>GAMETITVPTPIKQIFSDDAFAETIKDNLKKKSVTDAVTQNELNSIDQIIANNSDIKSVQGIQYLPNVTKLFLNGNKLTDIKPLANLKNLGWLFLDENKVKDLSSLKDLKKLKSLSLEHNGISDINGLVHLPQLESLYLGNNKITDITVLSRLTKLDTLSLEDNQISDIVPLAGLTKLQNLYLSKNHISDLRALAGLKNLDVLELFSQECLNKPINHQSNLVVPNTVKNTDGSLVTPEIISDDGDYEKPNVKWHLPEFTNEVSFIFYQPVTIGKAK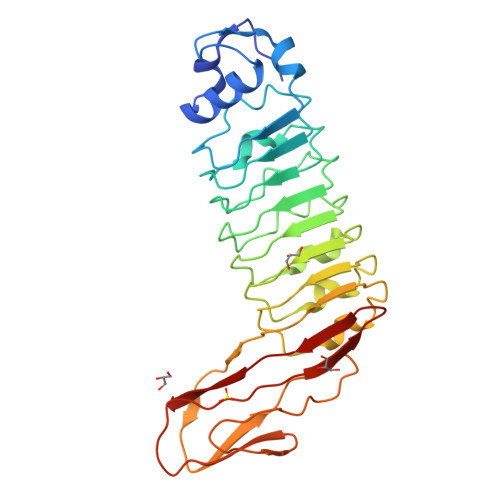ARFHGRVTQPLKE[6x]> SNAKNIEETELVVEEMLEQYPNGKIVRLLFHGEQAKLPIISHIVQEYQVEVSIIQGNIQQTKQGAVGSLYIQLL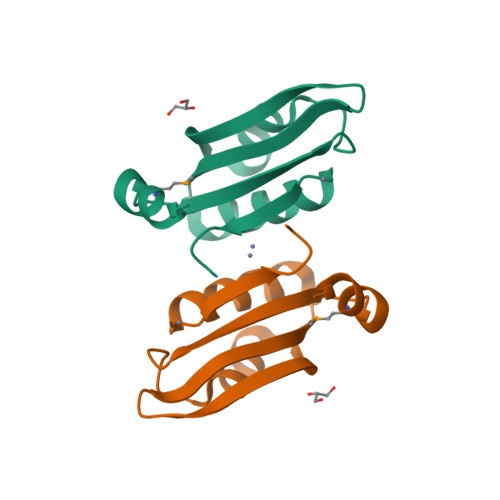GEEQNILAAIEGLRKLRVETEVIGNE>[12x]MTTVTSYPGVYIEELNSLALSVSNSATAVPVFAVDEQNQYISEDNAIRINSWMDYLNLIGNFNNEDKLDVSVRAYFANGGGYCYLVKTTSLEKIIPTLDDVTLLVAAGEDIKTTVDVLCQPGKGLFAVFDGPETELTINGAEEAKQAYTATPFAAVYYPWLKADWANIDIPPSAVMAGVYASVDLSRGVWKAPANVALKGGLEPKFLVTDELQGEYNTGRAINMIRNFSNTGTTVWGARTLEDKDNWRYVPVRRLFNSVERDIKRAMSFAMFEPNNQPTWERVRAAISNYLYSLWQQGGLAGSKEEDAYFVQIGKGITMTQEQIDAGQMIVKVGLAAVRPAEFIILQFTQDVEQR;>[12x]MSTSTSQIAVEYPIPVYRFIVSVGDEKIPFNSV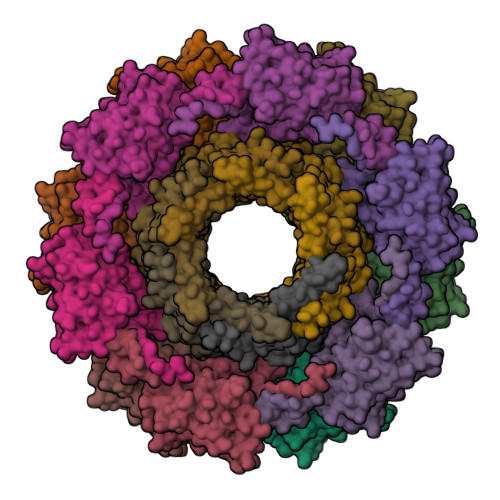SGLDISYDTIEYRDGVGNWFKMPGQSQSTNITLRKGVFPGKTELFDWINSIQLNQVEKKDITISLTNDAGTELLMTWNVSNAFPTSLTSPSFDATSNDIAVQEITLMADRVIMQAV> ADGIQSRKTYTLTDYLKNTYRLKLYSLRWISDHEYLYKQENNILVFNAEYGNSSVFLENSTFDEFGHSINDYSISPDGQFILLEYNYVKQWRHSYTASYDIYDLNKRQLITEERIPNNTQWVTWSPVGHKLAYVWNNDIYVKIEPNLPSYRITWTGKEDIIYNGITDWVYEEEVFSAYSALWWSPNGTFLAYAQFNDTEVPLIEYSFYSDESLQYPKTVRVPYPKAGAVNPTVKFFVVNTDSLSSVTNATSIQITAPASMLIGDHYLCDVTWATQERISLQWLRRIQNYSVMDICDYDESSGRWNCLVARQHIEMSTTGWVGRFRPSEPHFTLDGNSFYKIISNEEGYRHICYFQIDKKDCTFITKGTWEVIGIEALTSDYLYYISNEYKGMPGGRNLYKIQLSDYTKVTCLSCELNPERCQYYSVSFSKEAKYYQLRCSGPGLPLYTLHSSVNDKGLRVLEDNSALDKMLQNVQMPSKKLDFIILNETKFWYQMILPPHFDKSKKYPLLLDVYAGPCSQKADTVFRLNWATYLASTENIIVASFDGRGSGYQGDKIMHAINRRLGTFEVEDQIEAARQFSKMGFVDNKRIAIWGWSYGGYVTSMVLGSGSGVFKCGIAVAPVSRWEYYDSVYTERYMGLPTPEDNLDHYRNSTVMSRAENFKQVEYLLIHGTADDNVHFQQSAQISKALVDVGVDFQAMWYTDEDHGIASSTAHQHIYTHMSHFIKQCFSLPHHHHHH;> ADGIQEAKPSGSVVEQAEGVECDFSPLLSGTPPQVYNFKRLVFTNCNYNLTKLLSLFSVNDFTCSQISPAAIASNCYSSLILDYFSYPLSM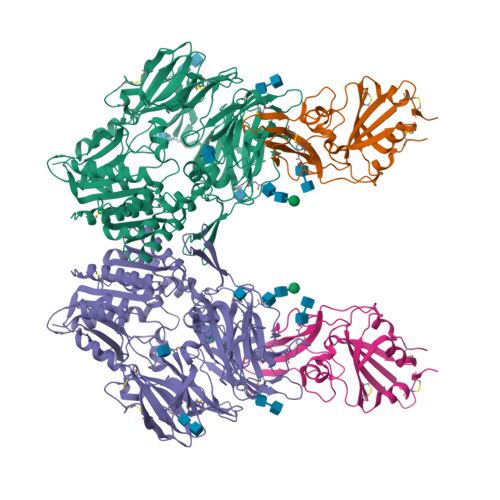KSDLSVSSAGPISQFNYKQSFSNPTCLILATVPHNLTTITKPLKYSYINKCSRLLSDDRTEVPQLVNANQYSPCVSIVPSTVWEDGDYYRKQLSPLEGGGWLVASGSTVAMTEQLQMGFGITVQYGTDTNSVCPKLEFANDTKIASQLGNCVEYHHHHHH>[2x]GSAPCLLKTKDWWTYEFCYGRHIQQYHMEDSEIKGEVLYLGYYQSAFDWDDETAKASKQHRLKRYHSQTYGNGSKCDLNGRPREAEVRF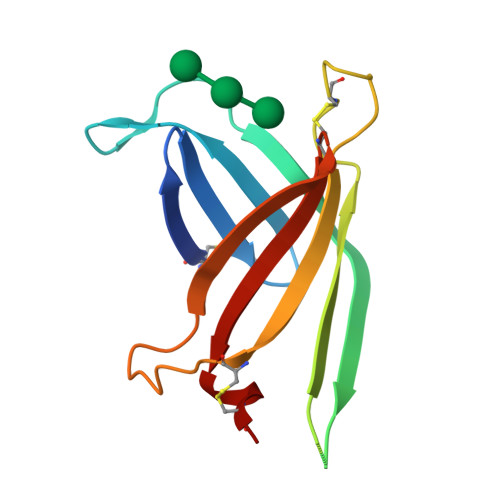LCDEGAGISGDYIDRVDEPLSCSYVLTIRTPRLCP Ngb is over-expressed in hypoxic conditions and it may be involved in gas/redox sensing, radical scavenging, and/or signal transduction. Notably, hexacoordination in Ngb accounts for a peculiar structural rearrangement and complex kinetics upon ligand binding, which takes place when the distal histidine (His(E7)64), engaged in internal iron hexacoordination, dissociates from the heme. The dissociation of His64 is the rate-limiting step for ligand binding and it triggers a repositioning of the heme which slides further inside a large internal cavity. In this study, we spectroscopically and structurally characterized three Ngb mutants aiming at pinpointing key features: a CD loop mutant with enhanced flexibility (Gly-loop), the F106A mutant and the double Gly-loop/F106A mutant.

The double conformation of the heme in 70:30 proportion, along with corresponding histidine double conformations, is present and His64(Nε)-Fe-His96(Nε) angles are unchanged with respect to WT. Besides some alternate conformations of the N- and C-termini, of the AB and EF loops, due to crystal packing changes, only the CD loop was significantly altered. Owing to the mutation of Tyr44 into a glycine, the propionate flips toward the proximal side of the heme, and the amino group of Lys67 is rotated by 180°. The absence of Tyr44, that is not pinning any more the loop to the heme, allows the displacement of Phe49 which might explain the D-helix destabilization. Quite surprisingly, the hydrophobic cluster involved in the support of the heme, and including the canonical Phe28(B10), Phe32(B14), Phe42(CD1) and Phe61(E4) is loosened in the Gly-loop mutant. As shown, in Fig. 4D, Phe42 and Phe61 are displaced with respect to the WT Ngb phenylalanine cluster: Phe42 is located about 0.6 Å further away from the heme (Cε(Phe42)-C3 methyl(heme) distance), whereas Phe61 is laterally shifted of approximately 2.4 Å (Cζ(Phe61 wt)-Cζ(Phe61 mutant) distance). The mobilization of the CD-loop-D-helix unit could facilitate the His64 dissociation from the heme iron, unlocking its swing-out displacement, thus leading to the increased CO binding velocities observed by rapid mixing.

> HMERPESELIRQSWRVVSRSPLEHGTVLFARLFALEPSLLPLFQGGGQFSSPEDSLSSPEFLDHIRKVMLVIDAAVTNVEDLSSLEEYLTSLGRKHRAVGVRLSSFSTVGESLLYMLEKSLGPDFTPATRTAWSRLYGAVVQAMSRGWDGE>MWVRGSGPSVLSRLQDAAVVRPGFLSTAEEETLSRELEPELRRRRYEYDHWDAAIHGFRETEKSRWSEASRAILRRVQAAAFGPGQTLLSSVHVLDLEARGYIKPHVDSIKFCGATIAGLSLLSPSVMRLVHTQEPGEWLELLLEPGSLYILRGSARYDFSHEILRDEESFFGERRIPRGRR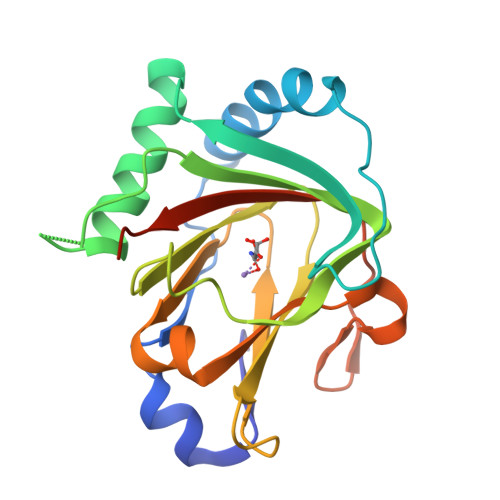ISVICRSLPEGMGPGESG[3x]>MRRNIFCLACLWIVQACLSLDRADILYNIRQTSRPDVIPTQRDRPVAVSVSLKFINILEVNEITNEVDVVFWQQTTWSDRTLAWNSSHSPDQVSVPISSLWVPDLAAYNAISKPEVLTPQLARVVSDGEVLYMPSIRQRFSCDVSGVDTESGATCRIKIGSWTHHSREISVDPTTENSDDSEYFSQYSRFEILDVTQKKNSVTYSCCPEAYEDVEVSLNFRKKGRSEIL[10x]

Neuronal nicotinic acetylcholine receptors (nAChRs) are pentameric ligand-gated ion channels present both in the central and peripheral nervous system. nAChRs belong to the Cys-loop superfamily and exist as homo or heteromeric receptors composed of either α subunits or α and β subunits in combination. The mulloskan AChBP is a structural and functional homologue of the extracellular domain of nAChRs. The erythrina alkaloid dihydro-β-erythroidine (DHβE) is a potent competitive antagonist at nAChRs that has been used extensively as a pharmacological tool compound to gain a better understanding of the involvement of these receptors in physiological processes. Each monomer consists of an N-terminal α-helix, two short α310 helices and a 10-stranded β-sandwich core.

In this study, we have determined the crystal structure of Ls-AChBP in complex with DHβE, which is a potent competitive antagonist of nAChRs. The crystal belongs to space group P212121 with a DHβE molecule bound at the interface of all ten monomers in the asymmetric unit of the crystal. The binding pocket is formed by the highly conserved aromatic residues Tyr89, Trp143, Tyr185, and Tyr192 from the principal side of the interface and Trp53 from the complementary side. The protonated tertiary nitrogen of DHβE lies within hydrogen-bonding distance of the backbone carbonyl of Trp143 (2.7 Å, chain D) and is also in close contact with the hydroxyl group of Tyr89 from the B-loop (3.5 Å, chain D). On the complementary side, DHβE interacts with the protein main chain via a water-mediated hydrogen bond. The oxygen of the methoxy group of DHβE accepts a hydrogen bond from a water molecule, which is tightly coordinated to the backbone carbonyl oxygen of Leu102 and nitrogen of Met114. In this way, the antagonist DHβE bridges the principal and complementary side of the interface in a way comparable to that of agonists. The structure reveals three main features that are unique to this antagonist: (i) DHβE introduces a C-loop closure compared to that of agonists, (ii) the C-loop undergoes a conformational shift perpendicular to the previously observed C-loop movements, and (iii) the hydrogen-bonding network of DHβE is similar to that of agonists. Thus, DHβE seems to prevent receptor activation via a mechanism different from that of prototypical antagonists and toxins.> SMVRGRISRLSVRDVRFPTSLGGHGADAMHTDPDYSAAYVVIETDAEDGIKGCGITFTLGKGTEVVVCAVNALAHHVLNKDLKDIVGDFRGFYRQLTSDGQLRWIGPEKGVVHLATAAVLNAVWDLWAKQEGKPVWKLLVDMDPRMLVSCIDFRYITDVLTEEDALEILQKGQIGKKEREKQMLAQGYPAYTTSCAWLGYSDDTLKQLCAQALKDGWTRFKVKVGADLQDDMRRCQIIRDMIGPEKTLMMDANQRWDVPEAVEWMSKLAKFKPLWIEEPTSPDDILGHATISKALVPLGIGIATGEQCHNRVIFKQLLQAKALQFLQIDSCRLGSVNENLSVLLMAKKFEIPVCPHAGGVGLCELVQHLII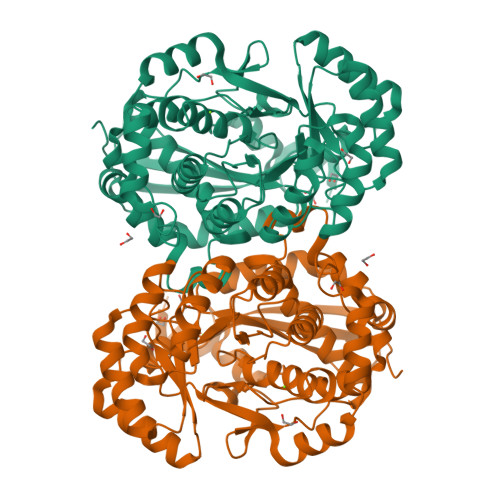FDYISVSASLENRVCEYVDHLHEHFKYPVMIQRASYMPPKDPGYSTEMKEESVKKHQYPDGEVWKKLLPA> APAANPAVTESVAPTTAPAPAAAAPESITPVNPAPTIQPPETRGMDLSIWGMYQHADAVVKAVMIGLVLASIVTWTILFAKGSELLRAKRRLRREQLALAEARSLDEASELAQNFSPESVSAVLLNDAQNELELSAESNDN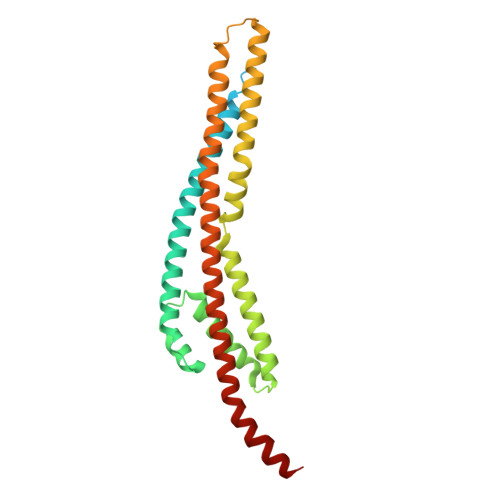NGIKERTGFRLERRVAAYSRNMGRGNGFLATIGAISPFVGLFGTVWGIMNSFIGIAHSQTTNLAVVAPGIAEALLATAMGLVAAIPAVVIYNIFARVISGHRAQVGDVAAQVLLLQGRDLDLAATAEAKRSQHAHQLRAG>TTNKPIVLSTWNFGLHANVEAWKVLSKGGKALDAVEKGVRLVEDDPTERSVGYGGRPDRDGRVTLDACIMDENYNIGSVACMEHIKNPISVARAVMEKKPHVMLVGDGALEFALSQGFKKENLLTAESEKEWKEWLKT[2x];>TIGMIALDAQGNLSGACTTSGMAYKMHGRVGDSPIIGAGLFVDNEIGAATATGHGEEVIRTVGTHLVVELMNQGRTPQQACKEAVERIVKIVNRRGKNLKDIQVGFIALNKKG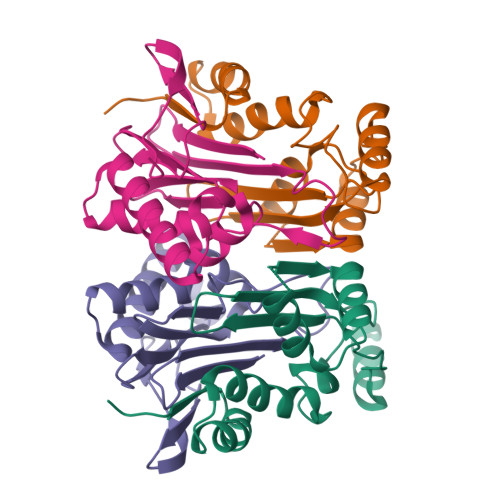EYGAYCIQDGFNFAVHDQKGNRLETPGFALK[2x]>[2x]MTGMSREEVESLIQEVLEVYPEKARKDRNKHLAVNDPAVTQSKKCIISNKKSQPGLMTIRGCAYAGSKGVVWGPIKDMIHISHGPVGCGQYSRAGQRNYYIGTTGVNAFVTMNFTSDFQEKDIVFGGDKKLAKLIDEVETLFPLNKGISVQSECPIGLIGDDIESVSKVKGAELSKTIVPVRCEGFRGVSQSLGHHIANDAVRDWVLGKRDEDTTFASTPYDVAIIGDYNIGGDAWSSRILLEEMGLRCVAQWSGDGSISEIELTPKVKLNLVHCYRSMNYISRHMEEKYGIPWMEYNFFGPTKTIESLRAIAAKFDESIQKKCEEVIAKYKPEWEAVVAKYRPRLEGKRVMLYIGGLRPRHVIGAYEDLGMEVVGTGYEFAHNDDYDRTMKEMGDSTLLYDDVTGYEFEEFVKRIKPDLIGSGIKEKFIFQKMGIPFREMHSWDYSGPYHGFDGFAIFARDMDMTLNNPCWKKLQAPWEASEGAEKVAASA;>[2x]MSQQVDKIKASYPLFLDQDYKDMLAKKRDGFEEKYPQDKIDEVFQWTTTKEYQELNFQREALTVNPAKACQPLGAVLCALGFEKTMPYVHGSQGCVAYFRSYFNRHFREPVSCVSDSMTEDAAVFGGQQNMKDGLQNCKATYKPDMIAVSTTCMAEVIGDDLNAFINNSKKEGFIPDEFPVPFAHTPSFVGSHVTGWDNMFEGIARYFTLKSMDDKVVGSNKKINIVPGFETYLGNFRVIKRMLSEMGVGYSLLSDPEEVLDTPADGQFRMYAGGTTQEEMKDAPNALNTVLLQPWHLEKTKKFVEGTWKHEVPKLNIPMGLDWTDEFLMKVSEISGQPIPASLTKERGRLVDMMTDSHTWLHGKRFALWGDPDFVMGLVKFLLELGCEPVHILCHNGNKRWKKAVDAILAASPYGKNATVYIGKDLWHLRSLVFTDKPDFMIGNSYGKFI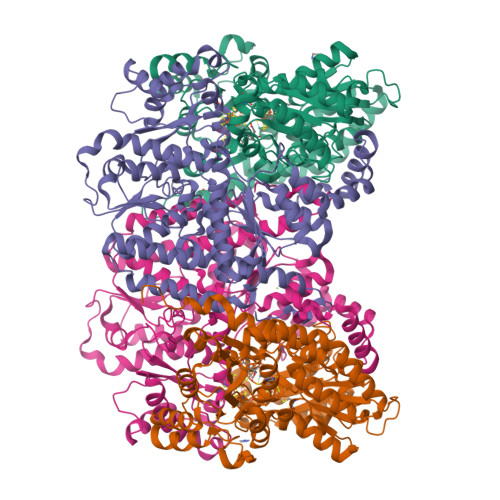QRDTLHKGKEFEVPLIRIGFPIFDRHHLHRSTTLGYEGAMQILTTLVNSILERLDEETRGMQATDYNHDLVR> AISDPKYSTVGFNIENSYDRLMKTIKEHKLKNYIKESV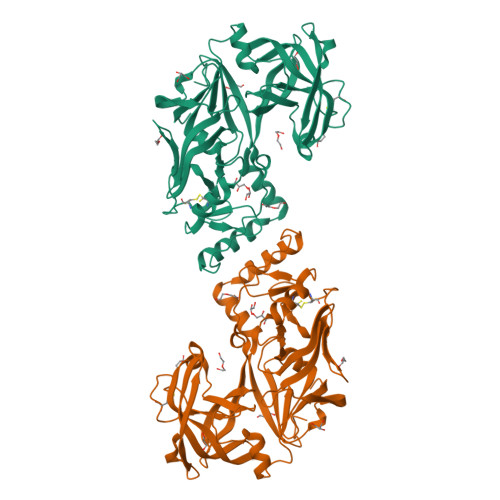KLFNKGLTKKSYLGSEFDNVELKDLANVLSFGEAKLGDNGQKFNFLFHTASSNVWVPSIKCTSESCESKNHYDSSKSKTYEKDDTPVKLTSKAGTISGIFSKDLVTIGKLSVPYKFIEMTEIVGFEPFYSESDVDGVFGLGWKDLSIGSIDPYIVELKTQNKIEQAVYSIYLPPENKNKGYLTIGGIEERFFDGPLNYEKLNHDLMWQVDLDVHFGNVSSKKANVILDSATSVITVPTEFFNQFVESASVFKVPFLSLYVTTCGNTKLPTLEYRSPNKVYTLEPKQYLEPLENIFSALCMLNIVPIDLEKNTFVLGDPFMRKYFTVYDYDNHTVGFALAKNL>MSSILRLDRLRQFIGELATLLDSRPDESTLLAQAHPLLAELVHQDDWLPEDCARPDPQRYQQYLLHVDSRQRFSVVSFVWGPGQITPVHDHRVWGLIGMLRGAEYSQPYAFDAGGRPHPSGARRRLEP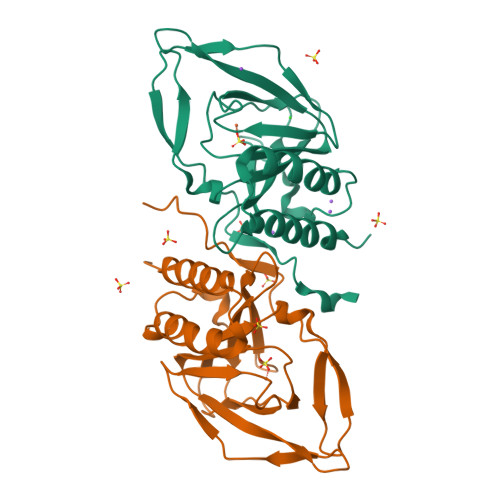GEVEALSPRIGDVHQVSNAFSDRTSISIHVYGANIGAVRRAVFSAEGEEKPFISGYSNSRLPNIWDLSKENPASAWSHPQFEK[2x]>MSPIHVRAHPGDVAERVLLPGDPGRAEWIAKTFLQNPRRYNDHRGLWGYTGLYKGVPVSVQTTGMGTPSAAIVVEELVRLGARVLVRVGTAGAASSDLAPGELIVAQGAVPLDGTTRQYLEGRPYAPV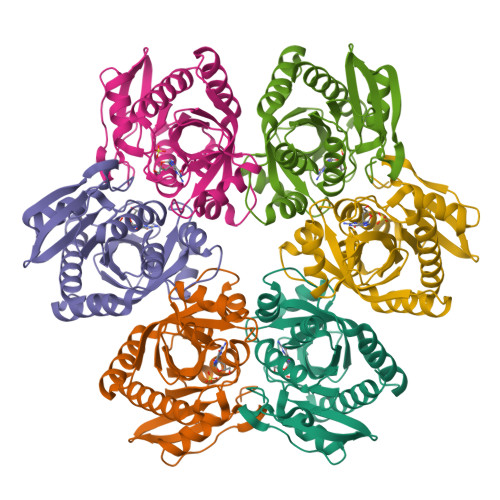PDPEVFRALWRRAEALGYPHRVGLVASEDAFYATTPEEARAWARYGVLAFEMEASALFLLGRMRGVRTGAILAVSNRIGDPELAPPEVLQEGVRRMVEVALEAVLEV[6x]> AKWVYKFEEGNASMRNLLGGKGCNLAEMTILGMPIPQGF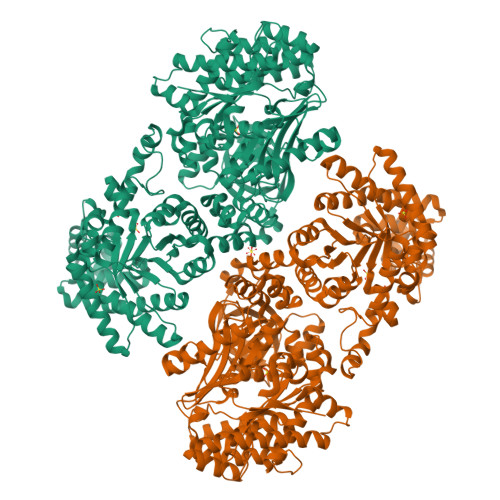TVTTEACTEYYNSGKQITQEIQDQIFEAITWLEELNGKKFGDTEDPLLVSVRSGARASMPGMMDTILNLGLNDVAVEGFAKKTGNPRFAYDSYRRFIQMYSDVVMEVPKSHFEKIIDAMKEEKGVHFDTDLTADDLKELAEKFKAVYKEAMNGEEFPQEPKDQLMGAVKAVFRSWDNPRAIVYRRMNDIPGDWGTAVNVQTMVFGNKGETSGTGVAFTRNPSTGEKGIYGEYLINAQGEDVVAGVRTPQPITQLENDMPDCYKQFMDLAMKLEKHFRDMQDMEFTIEEGKLYFLQTRNGKRTAPAALQIACDLVDEGMITEEEAVVRIEAKSLDQLLHPTFNPAALKAGEVIGSALPASPGAAAGKVYFTADEAKAAHEKGERVILVRLETSPEDIEGMHAAEGILTVRGGMTSHAAVVARGMGTCCVSGCGEIKINEEAKTFELGGHTFAEGDYISLDGSTGKIYKGDIETQEASVSGSFERIMVWADKFRTLKVRTNADTPEDTLNAVKLGAEGIGLCRTEHMFFEADRIMKIRKMILSDSVEAREEALNELIPFQKGDFKAMYKALEGRPMTVRYLDPPLHEFVPHTEEEQAELAKNMGLTLAEVKAKVDELHEFNPMMGHRGCRLAVTYPEIAKMQTRAVMEAAIEVKEETGIDIVPEIMIPLVGEKKELKFVKDVVVEVAEQVKKEKGSDMQYHIGTMIEIPRAALTADAIAEEAEFFSFGTNDLTQMTFGFSRDDAGKFLDSYYKAKIYESDPFARLDQTGVGQLVEMAVKKGRQTRPGLKCGICGEHGGDPSSVEFCHKVGLNYVSCSPFRVPIARLAAAQAALNNK> SLEKR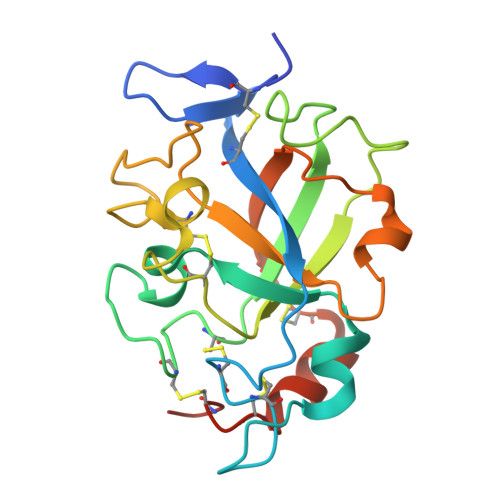AQLCQPDAHGVRRFNGRPCASTTRYVDGHKGACGCGQKGSDTPFPWNLQKHVTAPSERYFDDGGSNLWCGKNCGKCVRLTPTGGFVPGKGGAPPNHNPVVFMVTNACPINGNEEWCGISGKPGTNHVNSHGYEVHFDLQDQVGQVEALHWDNPEVTWEEVPCPGDLQANYQQCECHNSDHHHHHH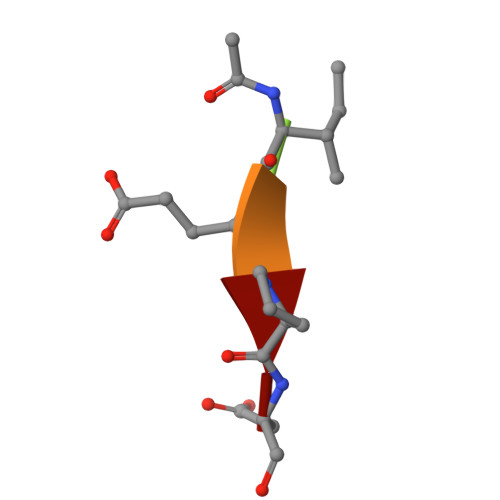> XIEPD>MGSITENTSWNKEFSAEAVNGVFVLCKSSSKSCATNDLARASKEYLPASTFKIPNAIIGLETGVIKNEHQVFKWDGKPRAMKQWERDLTLRGAIQVSAVPVFQQIAREVGEVRMQKYLKKFSYGNQNISGGIDKFWLEGQLRISAVNQVEFLESLYLNKLSASKENQLIVKEALVTEAAPEYLVHSKTGFSGVGTESNPGVAWWVGWVEKETEVYFFAFNMDIDNESKLPLRKSIPTKIMESEGIIG[2x]

pmcβ-Lactamases are a major mechanism of resistance to the clinically vital β-lactam antibiotics, with >2,000 different β-lactamases reported (1). β-Lactamases are grouped into classes A, C, and D, which employ a nucleophilic serine in catalysis (serine β-lactamases, SBLs), and class B, which employ metal ions in catalysis (2). Penam sulfones, which are structurally related to penicillins, inhibit clinically important serine β-lactamases (SBLs) by forming transiently stable covalent complexes, thereby protecting β-lactam antibiotics from hydrolysis. Oxidation of penams to their sulfone state promotes bifurcation of their reaction with SBLs at the acyl–enzyme stage to give transiently inactivating species that are more resistant to hydrolysis than the nascent AEC 2, turning penam sulfones into transient inactivators of SBLs. Studies on the mechanism of the new SBLi enmetazobactam employing mass spectrometry and X-ray crystallography inform on its mode of action and also lead to reevaluation of mechanisms of current clinically important SBLi.

Samples of OXA-10, treated with tazobactam or tazobactam in combination with BME (with full conversion to the respective −18- and +60-Da species verified by SPE-MS) were crystallized. Three high-resolution structures with two molecules in the asymmetric unit (ASU) were obtained, each using similar crystallization conditions. Evidence for cross-linking was observed in both OXA-10 chains. In chain A, clear and continuous electron density for both the Lal cross-link 10 and some unreacted carbamylated lysine was observed. The quality of the electron density map was overall less clear in chain B, though the mFo-DFc polder OMIT map indicates partial cross-linking. However, no clear density for the remaining carbamylated lysine was apparent in chain B, which was therefore not included in the final model. By contrast, with the D(2S)-stereochemistry observed on BME addition to Dha 9, the new chiral center formed by reaction of Lys70 with Dha 9 has, at least predominantly, the L(2S)-stereochemistry. The combined SPE-MS (including derivatization trials with BME), LC-MS/MS, and crystallographic results imply initial formation of a Dha residue 9, which reacts with Nε-amine of a Lys side chain to give the cross-linked Lal species 10. To date Lal 10 has rarely been identified in natural protein structures under biological conditions, with the spirochaete flagella hook protein being a notable example, and it has not previously been described with a β-lactamase. From the inhibition perspective, the Dha 9 and Lal cross-linked 10 species (which cannot be directly distinguished by intact protein MS) are of particular interest as they are the only modifications we observed leading to apparently irreversible inactivation of both class A and D SBLs.>GAMGSRKSKAELQSEERKRIDELIESGKEEGMKIDLIDGKGRGVIATKQFSRGDFVVEFHGDLIEITDAKKREALYAQDPSTGCYMYYFQYLSKTYCVDATRETNRLGRLINHSKCGNCQTKLHDIDGVPHLILIASRDIA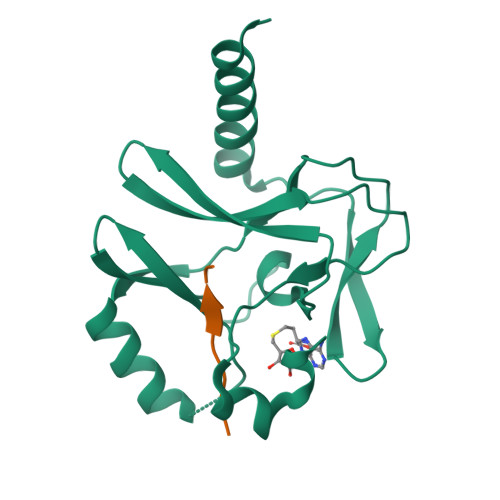AGEELLYDYGDRSKASIEAHPWLKH[4x];>[4x]AKRHRKVLRD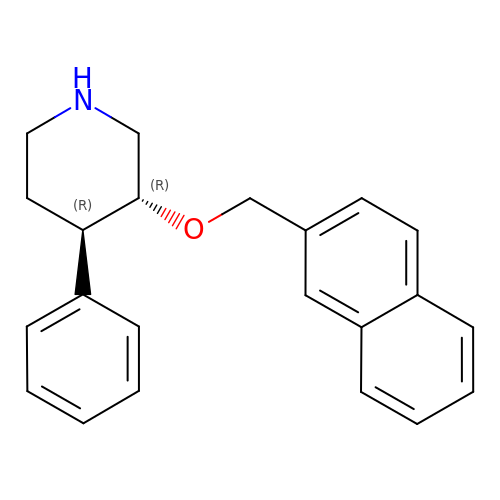(3R,4R)-3-(naphthalen-2-ylmethoxy)-4-phenylpiperidine | C22 H23 N O | CLTKEDPZPCYCIO-YADHBBJMSA-N> GPGSEFEPEKEEIRERYELSEKMLSACNLLKYNIKDPKALASKDMRICLNTLQHDWFRVSSQKSAVPAMVGDYIAAFEAVSPDVLRYIINMADGNGNTALHYSVSHSNFQIVKLLLDADVCNVDHQNKAGYTPIMLAALAAVEAEKDMQVVEELFSCGDVNAKASQAGQTALMLAVSHGR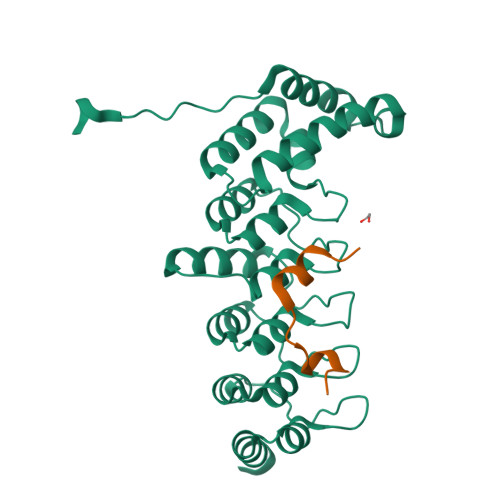IDMVKGLLACGADVNIQDDEGSTALMCASEHGHVEIVKLLLAQPGCNGHLEDNDGSTALSIALEAGHKDIAVLLYAHLNFSKAQSPSTPRLGRKTSPGPTHRGSFD;> PKNKARRRTTTQMELLYAD> AEQKTLHIYNWTDYIAPDTVANFEKETGIKVVYDVFDSNEVLEGKLMAGSTGFDLVVPSASFLERQLTAGVFQPLDKSKLPEWKNLDPELLKLVAKHDPDNKFAMPYMWATTGIGYNVDKVKAVLGENAPVDSWDLILKPENLEKLKSCGVSFLDDPEEVFATVLNYLGKDPNSTKADDYTGPATDLLLKLRPNIRYFHSSQYINDLANG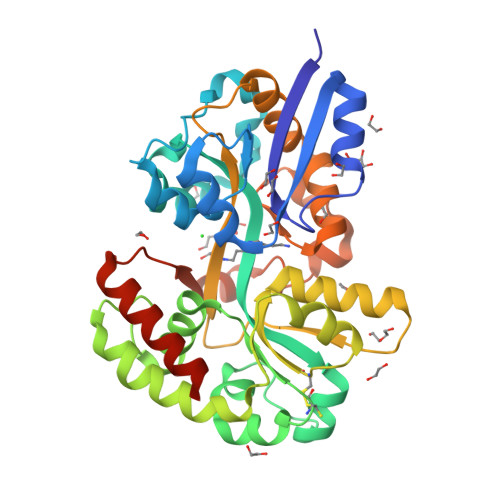DICVAIGWAGSVWQASNRAKEAKNGVNVSFSIPKEGAMAWFDVFAMPADAKNKDEAYQFLNYLLRPDVVAHISDHVFYANANKAATPLVSAEVRENPGIYPPADVRAKLFTQKVQDPKIDRVRTRAWTKVKSGKLEHHHHHH>[2x]MYGKIIFVLLLSEIVSISASSTTGVAMHTSTSSSVTKSYISSQTNDTHKRDTYAATPRAHEVSEISVRTVYPPEEETGERVQLAHHFSEPEITLIIFGVMAGVIGTILLISYGIRRLIKKSPSDVKPLPSPDTDVPLSSVEIENPETSDQ;>MEELQDDYEDMMEENLEQEEYEDPDIPESQMEEPAAHDTEATATDYHTTSHPGTHKVYVELQELVMDEKNQELRWMEAARWVQLEENLGENGAWGRPHLSHLTFWSLLELRRVFTKGTVLLDLQETSLAGVANQLLDRFIFEDQIRPQDREELLRALLLKHSHAGELEALGGVKPAVLTRSGDPSQPLLPQHSSLETQLFCEQGDGGTEGHSPSGILEKIPPDSEATLVLVGRADFLEQPVLGFVRLQEAAELEAVELPVPIRFLFVLLGPEAPHIDYTQLGRAAATLMSERVFRIDAYMAQSRGELLHSLEGFLDCSLVLPPTDAPSEQALLSLVPVQRELLRRRYQSSPAKPDSSFYKGLDLNGGPDDPLQQTGQLFGGLVRDIRRRYPYYLSDITDAFSPQVLAAVIFIYFAALSPAITFGGLLGEKTRNQMGVSELLISTAVQGILFALLGAQPLLVVGFSGPLLVFEEAFFSFCETNGLEYIVGRVWIGFWLILLVVLVVAFEGSFLVRFISRYTQEIFSFLISLIFIYETFSKLIKIFQDHPLQKTYNYNVLMVPKPQGPLPNTALLSLVLMAGTFFFAMMLRKFKNSSYFPGKLRRVIGDFGVPISILIMVLV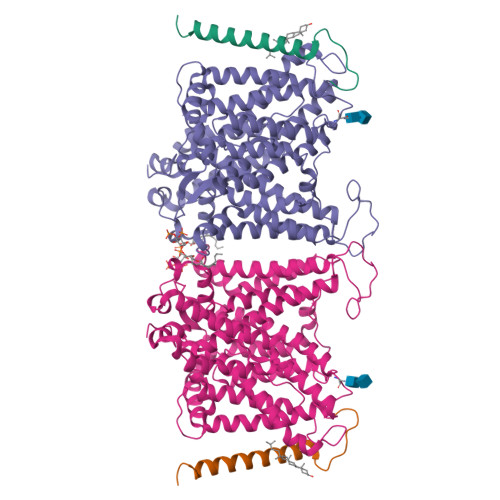DFFIQDTYTQKLSVPDGFKVSNSSARGWVIHPLGLRSEFPIWMMFASALPALLVFILIFLESQITTLIVSKPERKMVKGSGFHLDLLLVVGMGGVAALFGMPWLSATTVRSVTHANALTVMGKASTPGAAAQIQEVKEQRISGLLVAVLVGLSILMEPILSRIPLAVLFGIFLYMGVTSLSGIQLFDRILLLFKPPKYHPDVPYVKRVKTWRMHLFTGIQIICLAVLWVVKSTPASLALPFVLILTVPLRRVLLPLIFRNVELQCLDADDAKATFDEEEGRDEYDEVAMPV[2x]>[2x]MRFIHALLLAGIAHSAYASEK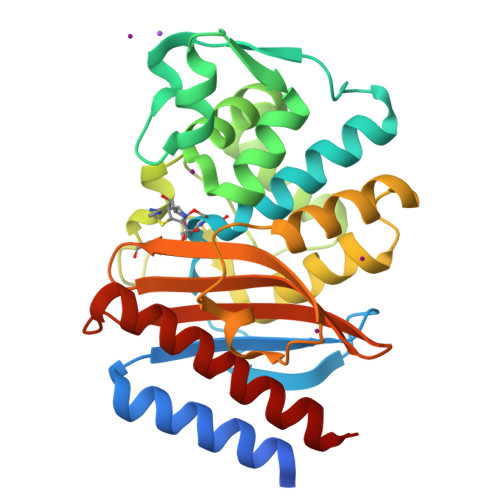LTFKTDLEKLEREKAAQIGVAIVDPQGEIVAGHRMAQRFAMCSTFKFPLAALVFERIDSGTERGDRKLSYGPDMIVEWSPATERFLASGHMTVLEAAQAAVQLSDNGATNLLLREIGGPAAMTQYFRKIGDSVSRLDRKEPEMGDNTPGDLRDTTTPIAMARTVAKVLYGGALTSTSTHTIERWLIGNQTGDATLRAGFPKDWVVGEKTGTCANGGRNDIGFFKAQERDYAVAVYTTAPKLSAVERDELVASVGQVITQLILSTDK> KKLIPILEKIPEVELPVKEITFKEKLKWTGIVLVLYFI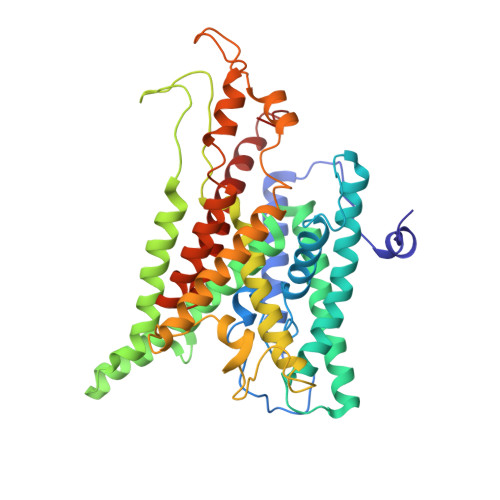MGCIDVYTAGAQIPAIFEFWQTITASRIGTLITLGIGPIVTAGIIMQLLVGSGIIQMDLSIPENRALFQGCQKLLSIIMCFVEAVLFVGAGAFGILTPLLAFLVIIQIAFGSIILIYLDEIVSKYGIGSGIGLFIAAGVSQTIFVGALGPEGYLWKFLNSLIQGVPNIEYIAPIIGTIIVFLMVVYAECMRVEIPLAHGRIKGAVGKYPIKFVYVSNIPVILAAALFANIQLWGLALYRMGIPILGHYEGGRAVDGIAYYLSTPYGLSSVISDPIHAIVYMIAMIITCVMFGIFWVETTGLDPKSMAKRIGSLGMAIKGFRKSAIEHRLKRYIPPLTVMSSAFVGFLATIANFIGALGGGTGVLLTVSIVYRMYEQLLREKVSELHPAIAKL> WQENKSWNAHFTEHKSQGVVVLWNENKQQGFTNNLKRANQAFLPAGTFKIPNSLIALDLGVVKDEHQVFKWDGQTRDIATWNRDHNLITAMKYSVVPVYQEFARQIGEARM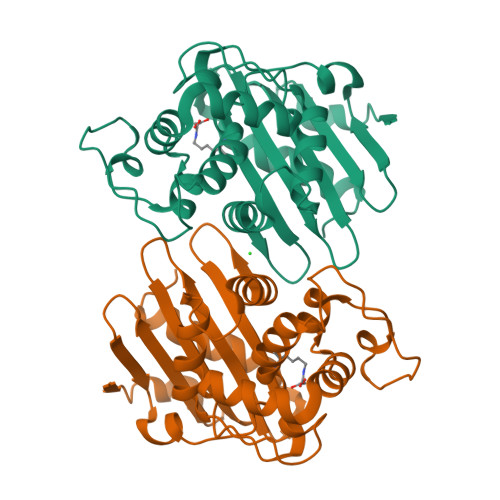SKMLHAFDYGNEDISGNVDSFWLDGGIRISATEQISFLRKLYHNKLHVSERSQRIVKQAMLTEANGDYIIRAKTGYDTKIGWWVGWVELDDNVWFFAMNMDMPTSDGLGLRQAITKEVLKQEKIIP N-{(1S)-2-(dimethylamino)-1-[3-methyl-5-(trifluoromethyl)phenyl]-2-oxoethyl}-4-[4-(trifluoromethyl)phenyl]pyridine-3-carboxamide | C25 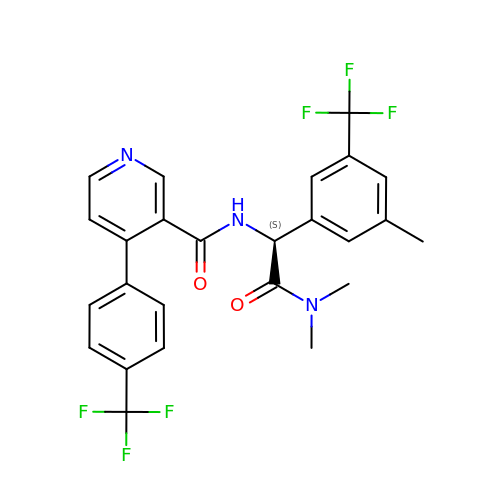H21 F6 N3 O2 | KPDNRBOZALCFHR-NRFANRHFSA-N benzyl 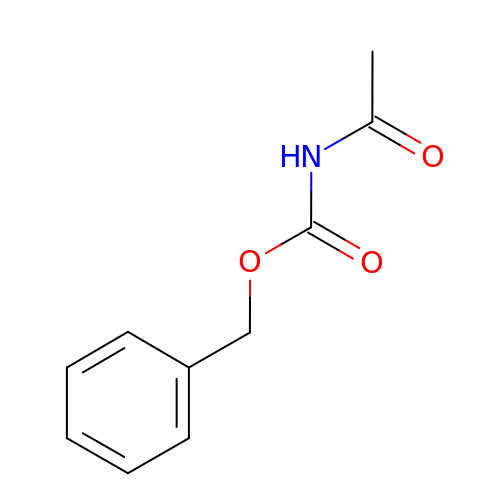acetylcarbamate | C10 H11 N O3 | IMSURJCYZMGADJ-UHFFFAOYSA-N> GSKAPPTFKVSLMDQSVREGQDVIMSIRVQGEPKPVVSWLRNRQPVRPDQRRFAEEAEGGLCRLRILAAERGDAGFYTCKAVNEYGARQCEARLEVRGE

The recently discovered Aortic Preferentially Expressed Protein-1 (APEG-1) may serve as a sensitive marker for vascular SMC differentiation. APEG-1 is expressed in differentiated vascular SMC in vivo and was found to be down-regulated rapidly in de-differentiated vascular SMC in vitro and in injured arteries in vivo. The amino acid sequence of APEG-1 (SwissProt Q15772) defines a single Ig-like domain. The structure of APEG-1 shows the intermediate set (I set) immunoglobulin superfamily fold which consists of a β-sandwich forming a central hydrophobic core.

Good quality crystals that were suitable for X-ray crystallographic studies were obtained following the truncation of the 14 N-terminal amino acids of APEG-1, a region predicted to be disordered. The X-ray structure of ΔAPEG-1 was determined and was refined to sub-atomic resolution (0.96 Å). The main hydrophobic core of the domain is formed around the aromatic residues W53, F22 and Y91. A disulfide linkage is normally present in extracellular immunoglobulin domains between strands B and F. In ΔAPEG-1 this is replaced by hydrophobic interactions between residues I41 and C93 in strands B and F, respectively. Only one cysteine of this bridge is present in ΔAPEG-1 and no disulfide linkages were found. The RGD motif folds into a 310 helix that is involved in the formation of a homodimer in the crystal which is mainly stabilized by salt bridges. The homodimer with the largest buried surface area utilizes end-to-end packing with the subunits' N-termini pointing in opposite directions. The residues involved in formation of this dimer are exclusively located within the loop cluster between strands CC', C'D and EF which lie close to the C-terminus and within the 310 helix which contains the RGD motif. The dimer interface includes two buried bi-dentate salt bridges – involving the RGD motif – between R65-D87 and R65'-D87' (the apostrophe denotes the adjacent ΔAPEG-1 molecule). An average dimer dissociation constant of Kd = 20 μM derived from the concentration-dependent Mw measurements was obtained for both full-length APEG-1 and ΔAPEG-1 at 100 mM NaCl, demonstrating the nearly identical amount of dimers.>[2x]MRDHRKIGKQLDLYHMQEEAPGMVFWHNDGWTIFRELEVFVRSKLKEYQYQEVKGPFMMDRVLWEKTGHWDNYKDAMFTTSSENREYCIKPMNCPGHVQIFNQGLKSYRDLPLRMAEFGSCHRNEPSGSLHGLMRVRGFTQDDAHIFCTEEQIRDEVNGCIRLVYDMYSTFGFEKIVVKLSTRPEKRIGSDEMWDRAEADLAVALEENNIPFEYQLGEGAFYGPKIEFTLYDCLDRAWQCGTVQLDFSLPSRLSASYVGEDNERKVPVMIHRAILGSMERFIGILTEEFAGFFPTWLAPVQVVIMNITDSQSEYVNELTQKLSNAGIRVKADLRNEKIGFKIREHTLRRVPYMLVCGDKEVESGKVAVRTRRGKDLGSMDVNEVIEKLQQEIRSRSLKQLEELEHHHHHH

ThrRS is one of the 20 (in general) aminoacyl-tRNA synthetases (AARSs) that are essential enzymes responsible for charging corresponding amino acids to their cognate tRNAs and providing the correct substrates for high-fidelity protein synthesis. We determined the crystal structures of both human and E. coli ThrRS in complex with BN, and identified a unique structural inhibition mechanism of BN against ThrRS. BN occupies a significant fraction of the total volume of the ThrRS enzymatic pocket, physically excluding all three of the physiological substrates of ThrRS, namely L-threonine (L-Thr), ATP and tRNA. Although occupying the canonical active site cavity, BN also extends into a fourth ‘orthogonal’ pocket.

We also crystallized an E. coli ThrRS fragment containing the catalytic and anticodon-binding domains with BN. Consistent with the 48% sequence identity between human and E. coli ThrRS’s in the catalytic domain, BN is bound in the active site cavity with a nearly identical structure in human and E. coli ThrRS–BN complex structures. The r.m.s.d. of all 35 non-hydrogen atoms of the bound BNs from the two structures is only 0.314 Å. We investigated whether BN induces such a state by comparing the E. coli ThrRS–BN structures with those of canonical ligands: L-Thr26, ATP35 and AMP together with tRNA27. By comparison with all three standard aminoacylation substrates, L-Thr, ATP, and AMP+tRNAThr, BN is inserted 4 Å deeper into the active site cleft. The additional interactions associated with the deeper binding lead to a significant conformational opening at the upper side of active site, thus highlighting an induced-fit component to the binding mechanism of BN. This upper active site opening also distinguishes the ThrRS–BN complex from the comparatively modest conformational change observed when ThrRS is bound to its aminoacylation substrates. In our structures, a major feature of the BN-induced conformational change is a 14° rotation of the α helix comprised by residues 431–448 that produce a 10-Å displacement of the preceding loop. This structural change is observed in both the human and E. coli ThrRS–BN complexes. In support of the discriminative role of these residues, mutations at H309 and L489 in E. coli ThrRS (corresponding to H388 and L567 in human) confer 300- to 1,000-fold increases in Ki, representing significant resistance to BN20.> MISLSDIENLIQHIWEEPIFSDVTSKKVVVSLY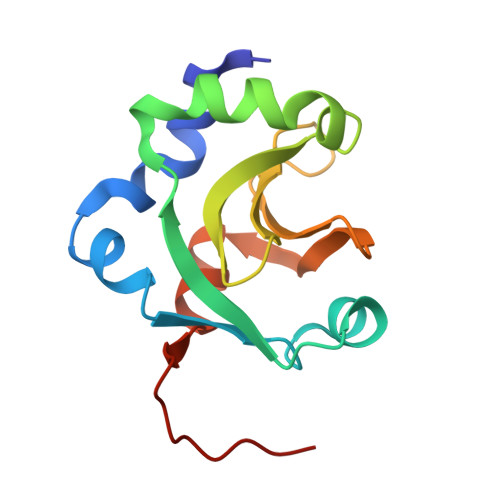GTLSKKIPDKFIIIEEVFPKDELEDIWSNYEEYLDEYLIFPFLGTLGEAVICIGYGNDNKGKIFYFDFDFGACELDGDNLEAFLEKLLESGSTENLYFQ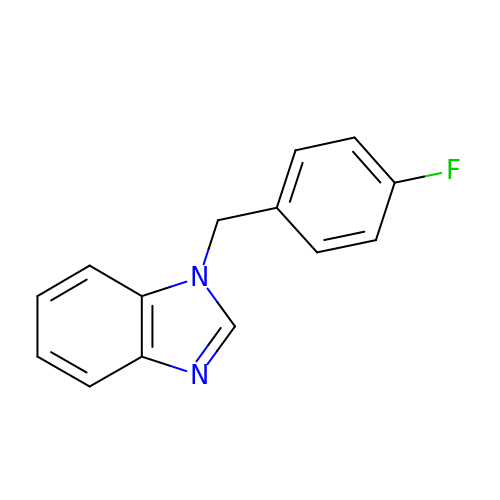1-[(4-fluorophenyl)methyl]benzimidazole | C14 H11 F N2 | QLQZBMMYHJKDSH-UHFFFAOYSA-N>PMTLGYWNIRGLAHSIRLLLEYTDSSYEEKKYTMGDA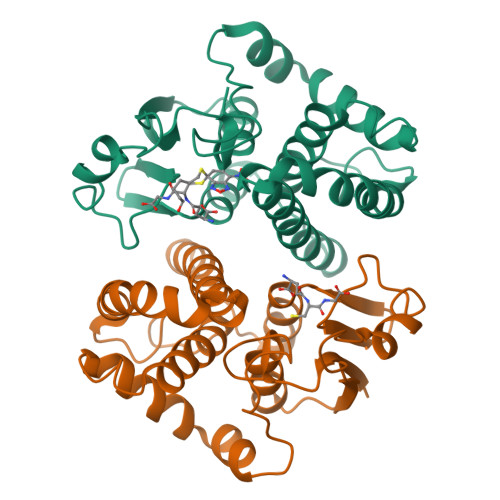PDYDRSQWLNEKFKLGLDFPNLPYLIDGTHKITQSNAILRYIARKHNLCGESEKEQIREDILENQFMDSRMQLAKLCYDPDFEKLKPEYLQALPEMLKLYSQFLGKQPWFLGDKITFVDFIAYDVLERNQVFEPSCLDAFPNLKDFISRFEGLEKISAYMKSSRFLPRPVFTKMAVWGNK[4x]>NUNGACUUAAGUCG[2x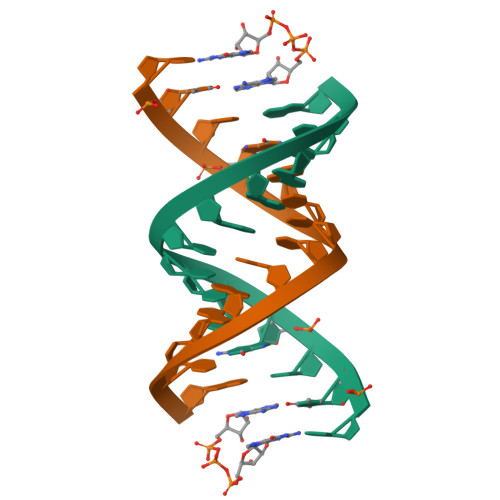]>SNAMSLKDYDAARLAQVREEVTAKYAELKAKNLSLDLTRGKPSAEQLDLSNDLLSLPGGDFRTKDGVDCRNYGGLLGIADIRELWAEALGLPADLVVAQDGSSLNIMFDLISWSYTWGNNDSSRPWSAEEKVKWLCPVPGYDRHFTITEHFGFEMINVPMTDEGPDMGVVRELVKDPQVKGMWTVPVFGNPTGVTFSEQTCRELAEMSTAAPDFRIVWDNAYALHTLSDEFPIVHNVIEFAQAAGNPNRFWFMSSTSKITHAGSGVSFFASSKENIEWYASHA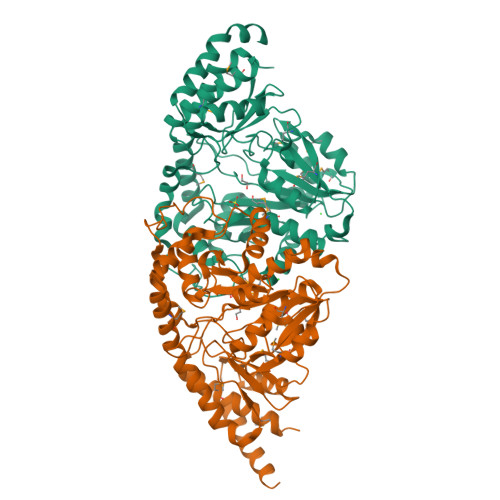NVRGIGPNKLNQLAHAQFFGDVAGLKAHMLKHAASLAPKFERVLEILDSRLSEYGVAKWTSPTGGYFISVDVVPGTASRVVELAKEAGIALTGAGSSFPLHNDPNNENIRLAPSLPPVAELEVAMDGFATCVLMAALEV[4x]>MKIRVADEKELPMILQFLTEVKAYMDVVGITQWTKDYPSQGDIQEDITKKRLYLLVHEEMIFSMATFCMEQEQDFVWLKRFATSPNYIAKGYGSLLFHELEKRAVWEGRRKMYA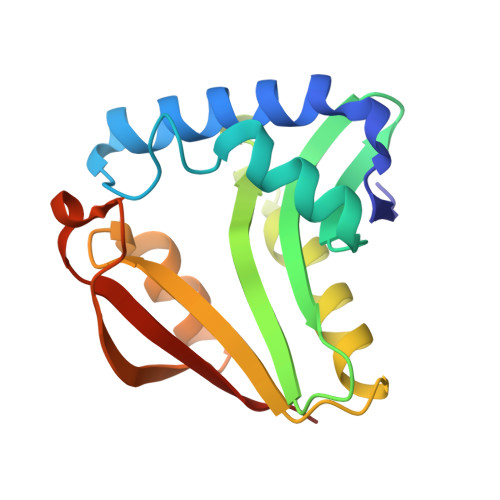QTNHTNHRMIRFFESKGFTKIHESLQMNRLDFGSFYLYVKELENQSIV[2x]>[2x]MSAIENFDAHTPMMQQYLRLKAQHPEILLFYRMGDFYELFYDDAKRASQLLDISLTKRGASAGEPIPMAGIPYHAVENYLAKLVNQGESVAIAEQIGDPATSKGPVERKVVRIVTPGTISDEALLQERQDNLLAAIWQDSKGFGYATLDISSGRFRLSEPADRETMAAELQRTNPAELLYAEDFAEMSLIEGRRGLRRRPLWEFEIDTARQQLNLQFGTRDLVGFGVENAPRGLSAAGALLQYAKCTQRTTLPHIRSITMEREQDSIIMDAATRRNLEITQNLAGGAENTLASVLDSTVTPMGSRMLKRWLHMPVRDTRVLLERQQTIGALQDFTAGLQPVLRQVGDLERILARLALRTARPRDLARMRHAFQQLPELR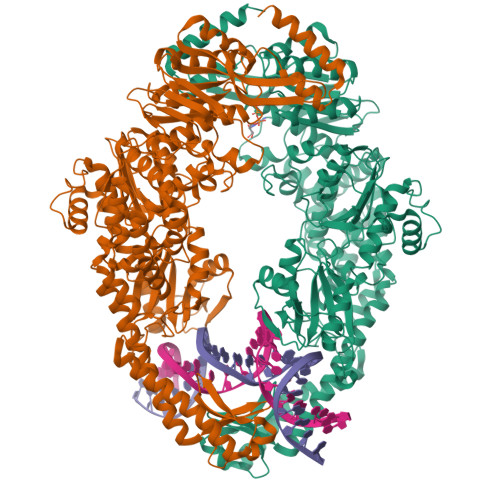AQLETVDSAPVQALREKMGEFAELRDLLERAIIDTPPVLVRDGGVIASGYNEELDEWRALADGATDYLERLEVRERERTGLDTLKVGFNAVHGYYIQISRGQSHLAPINYMRRQTLKNAERYIIPELKEYEDKVLTSKGKALALEKQLYEELFDLLLPHLEALQQSASALAELDVLVNLAERAYTLNYTSPTFIDKPGIRITEGRHPVVEQVLNEPFIANPLNLSPQRRMLIITGPNMGGKSTYMRQTALIALMAYIGSYVPAQKVEIGPIDRIFTRVGAADDLASGRSTFMVEMTETANILHNATEYSLVLMDEIGRGTSTYDGLSLAWAVAENLANKIKALTLFATHYFELTQLPEKMEGVANVHLDALEHGDTIAFMHSVQDGAASKSYGLAVAALAGVPKEVIKRARQKLRELESISPNAAATQVDGTQMSLLSVPEETSPAVEALENLDPRSLTPRQALEWIYRLKSLV> MNEHYTESDIKRNHKTEKNKTEKEKFKDSINNLVKTEFTNETLDKIQQTQDLLKKIPKDVLEIYSELGGEIYFTDIDLVEHKELQDLSEEEKNSMNSRGEKVPFASRFVFE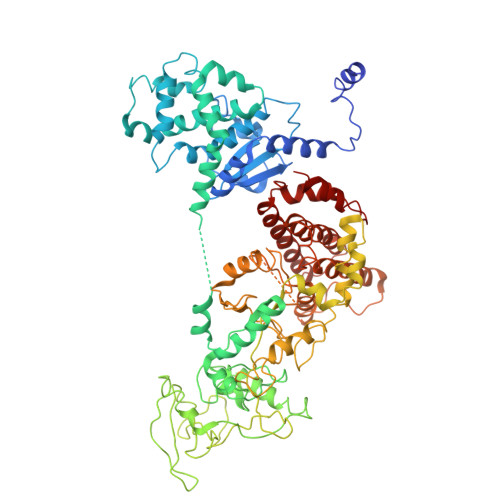KKRETPKLIINIKDYAINSEQSKEVYYEIGKGISLDIISKDKSLDPEFLNLIKSLSDDSDSSDLLFSQKFKEKLELNNKSIDINFIKENLTEFQHAFSLAFSYYFAPDHRTVLELYAPDMFEYMNKLEKGGFEKISESLKKEGVEKDRIDVLKGEKALKASGLVPEHADAFKKIARELNTYILFRPVNKLATNLIKSGVATKGLNVHGKSSDWGPVAGYIPFDQDLSKKHGQQLAVEKGNLENKKSITEHEGEIGKIPLKLDHLRIEELKENGIILKGKKEIDNGKKYYLLESNNQVYEFRISDENNEVQYKTKEGKITVLGEKFNWRNIEVMAKNVEGVLKPLTADYDLFALAPSLTEIKKQIPQKEWDKVVNTPNSLEKQKGVTNLLIKYGIERKPDSTKGTLSNWQKQMLDRLNEAVKYTGYTGGDVVNHGTEQDNEEFPEKDNEIFIINPEGEFILTKNWEMTGRFIEKNITGKDYLYYFNRSYNKIAPGNKAYIEWTDPITKAKINTIPTSAEFIKNLSSIRRSSNVGVYKDSGDKDEFAKKESVKKIAGYLSDYYNSANHIFSQEKKRKISIFRGIQAYNEIENVLKSKQIAPEYKNYFQYLKERITNQVQLLLTHQKSNIEFKLLYKQLNFTENETDNFEVFQKIIDEK>[2x]QFQKPGDAIEYRQSAFTLIANHFGRVAAMAQGKAPFDAKVAAENIALVSTLSKLPLTAFGPGTDKGHGTEAKPAVWSDAAGFKAAADKFAAAVDKLDAAGKTGDFAQIKAAVGETGGACK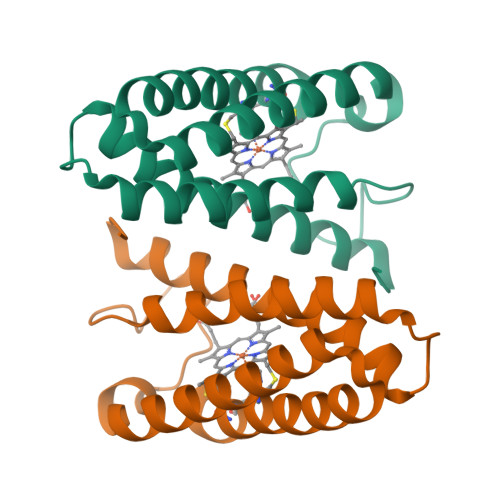GCHDKFKEK>[6x]MQIDAVKCATASRNTFNFMIKNIIPNKSIILMKKVYELTSEEALSYFLRHDSYTTLELPAYINFTTLLNDINSSIHNKKIKIEPTAKELMGKDINYEVLVSKDGLYSWRRITLINPLYYVYFCRKITAPATWEIITEKFKSFESNDLFTCSSIPVRKDNSSNIAASVMNWWEDFEQKSLALALEYEFMFSTDISNFYPSIYTHSFEWVFISKEEAKKKKSKNNPGGLIDSHIQMMMNNQTNGIPLGSTLMDTFAELILGQIDIELRKKTNELKIINYKVVRYRDDYRIFSNSKDDLDIISKCLVNVLGDFGLDLNSKKTELYEDIILHSLKQAKKDYIKEKRHKSLQKMLYSIYLFSLKHPNSKTTVRYLNDFLRNLFKRKTIKDNGQQVDAMLGIISSIMAKNPTTYPVGTAIFSKLLSFLYGDDTQKKLTKLEQLHKKLDKQPNTEMLDIWFQRTQAKINLEWNKSYKSALCVRINDELTKEKTFSVNNLWNIDWIQGKETSPNKAKILSLLRKTKIVDTDKFDKMDDNITPEEVNLFF

Abortive infection (Abi) is a bacterial antiphage defense strategy involving suicide of the infected cell. Some Abi pathways involve polymerases that are related to reverse transcriptases. They are unique in the way they combine the ability to synthesize DNA in a template-independent manner with protein priming. Here, we report crystal and cryo-electron microscopy structures of two Abi polymerases: AbiK and Abi-P2. Both proteins adopt a bilobal structure with an RT-like domain that comprises palm and fingers subdomains and a unique helical domain.

We also obtained Abi-P2 crystals that diffracted X-rays to 3.1 Å. The crystal structure was solved by molecular replacement using the low resolution cryo-EM map. In the crystal structure of Abi-P2, no electron density was observed for the DNA, in agreement with the low Abs260/Abs280 ratio for this protein after purification. Abi-P2 adopts a trimeric arrangement that is similar to Ll-AbiK. The asymmetric unit for the crystal structure contained six protein molecules that were arranged similarly to Ll-AbiK hexamers as two trimers stacked back-to-back. Therefore, Abi-P2 also has the potential to adopt a hexameric architecture. The absence of DNA in the structure precluded identification of the tyrosine residue that is responsible for polymerization initiation. Two tyrosine residues (Tyr46 and Tyr61) are present in the region of Abi-P2 that corresponds to the region of AbiK that comprises its priming tyrosine. We individually substituted these two tyrosines with phenylalanine. The Y46F variant retained wild-type levels of activity, whereas the Y61F variant did not polymerize DNA, showing that the hydroxyl group of the latter residue is involved in DNA synthesis priming.>MSLNIKEASEKSGVSADTIRYYERIGLIPPIHRNESGVRKFGAEDLRWILFTRQMRRAGLSIEALIDYLALFREGEHTLEARAELLKKQRIELKNRIDVMQEALDRLDFKIDNYDTHLIPAQEELKDFN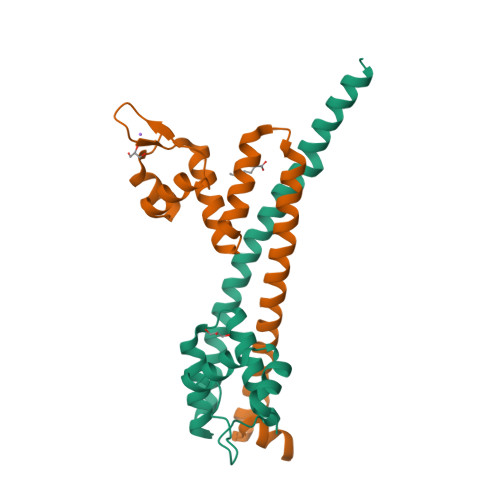VERSNEGHHHHHH[2x]> MRRSGRGSAVRWSSLCKCQCCLYRTPLGGTYFEQALPRSLGARQGKGVLSTVNTALSRKALKRRQSLPRKKLNVPLTAEGLKERLKQLSAEERELSIKNNTEECDEPSPNEFTTTHEARVALARVLHHGENAGERKEVAMRIPSFCRSPAVSETQSIVVDDKEGDITNAAVHVGCSVLGSDLDHLERDMIRDYHQRGKKLPTFDNIYRTLGCGRKGTSVSDTEPEDENSSGAIQSECGLGDAGRRGTVVVAPSHLHHSTPPTKGRSGEEEEEGGCFDTNTLPADANPHFPPGACDNEVLAPLSGGCA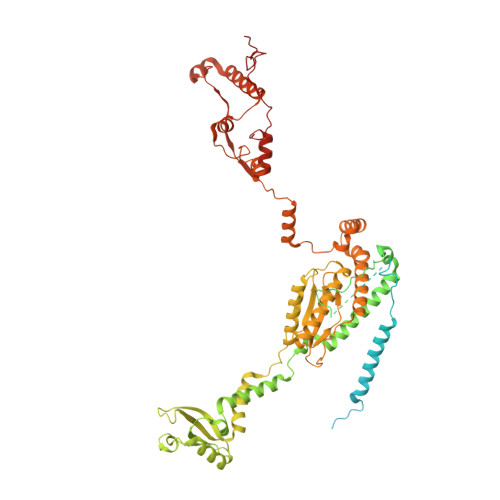ASEQTEITDTASFIPSNSRLSTAVYDAYRQRPADDRLVVLRGTDFWDNEENRARLQELTDYAEEDFAREMLMEGAMDTSEVGYSTNKVRKETLLYFQAHPINEMIQEPFARVRSILPSDGGPEVHFPADDPDTDVDIPTAQARTMARELGLDLIRVGTLYTPINDRRVVAVCTIADHREHMRDMIRFKIKKLGVQRPPTKEGIEVPFRGGTHPHAVRFKSIGIAKHLLLGHVVRINLTDFGTVREGFPVFGSILDEVARQALQLHAYHTAGVVRANYNEVYCYLYPSTGRSPKSTVLHPTQEQLATVRDRCLLEREREVYFDGLYDKKTPRERLTYMRKLQDGTAWADRDDGLSLQRQRDMKVMLGYLPKGNHELYAARGDVNVPAPFRASHPTSVDRWTHPQESNLEQAARGSAVLAKRLSMTVSEMHDRQETAENPATLDRFYYRIQGPALEAGELKEALGLKGNRKRLPRRAPGWATLGMEKVSPQEPGHAAK WW domains organize molecular assemblies by binding to short, proline rich peptide motifs each with ~4–6 residues. The type I WW domains bind to a consensus ‘PPxY’ motif (where P is proline, x is any amino acid and Y is tyrosine, also known as PY-motif) with very modest affinities (with Kd in the range of a few to a few tens of µM). To achieve this goal, we determined the high resolustion structures of 7 representative WW tandem/target complexes, and measured the binding constants of >100 WW domain tandems or isolated WW domains binding to known or previously unknown targets. In this study, we discovered that WW tandems, but not individual WW domains, can bind to target proteins with extremely high affinity and with very high sequence specificity.

Similar to the two PY-motifs of Dendrin that are separated by only two residues, the first two PY-motifs of PTPN14 are also next to each other with only two residues in between, and the PY12 motif sequence is evolutionarily conserved. We found that the KIBRA WW tandem also binds to PTPN14 PY12 with a super strong affinity (Kd ~8.2 nM). We further showed that KIBRA WW1 had a very weak binding to PTPN14 PY12 (Kd ~32 μM) and KIBRA WW2 had no detectable binding to PTPN14 PY12. Taken together, the above biochemical study revealed that the KIBRA WW tandem, via synergistic binding to the two PY-motifs immediately next to each other (i.e. PY12), can form a very tight complex with PTPN14. We solved the high-resolution crystal structures of KIBRA WW tandems in complex with PTPN14 PY12, AMOT PY34 and LATS1 PY23. A residue in the PY-motif linker (R440 in PTPN14, Q282 in AMOT and G553 in LATS) uses its carbonyl group to form a hydrogen-bond with the sidechain of Trp34. The sidechain of R440 of PTPN14 also forms charge-charge interactions with D17 and D19 in β12 loop of WW1. Substitution of R440 with Ala weakened PTPN14’s binding to KIBRA by 17-fold. Second, the C-terminal extension of PTPN14 PY12 tandem enhances its binding to KIBRA WW tandem by forming hydrophobic interactions with its WW1 domain. However, substitutions of the Pro residue with Cys, Ala, Ser, Thr, and Val lead to only mild weakening of the binding, whereas substitutions with bulky hydrophobic Leu, Met and Ile essentially disrupted the binding. The above results can be rationalized by the structure of the KIBRA WW tandem in complex with PTPN14 PY12 showing that the pocket accommodating the residue (T442 in Figure 6A) is quite small. The extensive interactions between the inter-domain linker and the C-terminal helix couples the two WW domain into a structural supramodule in these WW tandems, thus providing a structural and thermodynamic basis for highly synergistic bindings to target proteins. For example, the formation of the WW tandem supramodule allowed KIBRA WW12 to bind to PTPN14 with an ~3900 fold higher affinity when compared to the isolated WW domains (Figure 4D1 and Figure 1—figure supplement 1B and C).

> GPGSEFELPLPEGWEEARDFDGKVYYIDHRNRTTSWIDPRDRYTKPLTFADCISDELPLGWEEAYDPQVGDYFIDHNTKTTQIEDPRVQWRREQEHMLKDYLVVAQEALSAQKEIYQVKQQRLELAQQEYQQLH;> GPGSSHRHSAIIVPSYRPTPDYETVMRQMKRG> AEVCYSHLGCFSDEKPWAGTSQRPIKSLPSDPKKINTRFLLYTNENQNSYQLITATDIATIKASNFNLNRKTRFIIHGFTDSGENSWLSDMCKNMFQVEKVNC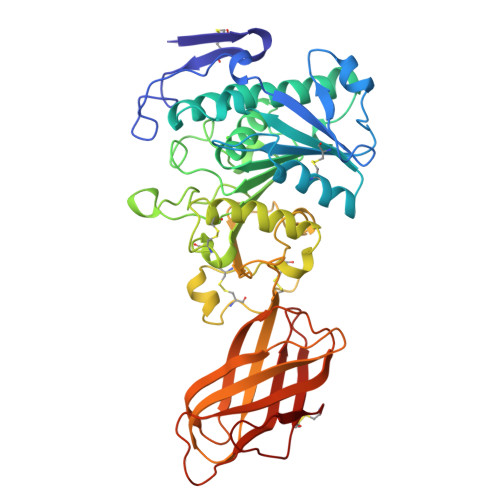ICVDWKGGSKAQYSQASQNIRVVGAEVAYLVQVLSTSLNYAPENVHIIGHSLGAHTAGEAGKRLNGLVGRITGLDPAEPYFQDTPEEVRLDPSDAKFVDVIHTDISPILPSLGFGMSQKVGHMDFFPNGGKDMPGCKTGISCNHHRSIEYYHSSILNPEGFLGYPCASYDEFQESGCFPCPAKGCPKMGHFADQYPGKTNAVEQTFFLNTGASDNFTRWRYKVSVTLSGKKVTGHILVSLFGNKGNSKQYEIFKGTLKPDSTHSNEFDSDVDVGDLQMVKFIWYNNVINPTLPRVGASKIIVETNVGKQFNFCSPETVREEVLLTLTPC Microbial rhodopsins that are extremely distantly related to animal visual rhodopsins comprise an expansive family of seven transmembrane proteins that contain a covalently attached cofactor, retinal. Upon absorption of a photon, retinal isomerizes triggering a series of structural transformations that correlate with functional and spectral changes and are known as the photocycle. Here we present a structural and functional characterization of Organic Lake Phycodnavirus rhodopsin II (OLPVRII), a representative of the second group of viral rhodopsins. Examination of the crystal structure, functional characterization and molecular dynamics (MD) simulations suggest that OLPVRII is a pentameric light-gated channel that is functionally analogous to well-studied pentameric ligand-gated ion channels playing crucial roles in many cellular processes.

The crystals diffracted up to 1.9 Å, and the structure of OLPVRII was solved at 1.9 Å. OLPVRII asymmetric unit cell contains five molecules of the protein organized in a pentamer with a bottle-like pore in the centre that has a narrow neck in the cytoplasmic part. Similarly to other microbial rhodopsins, each protomer of OLPVRII is organized as a bundle of seven transmembrane helices (A−G) connected by relatively short loops. The retinal cofactor is covalently bound to Lys195 through the Schiff base (RSB), and the electron densities indicate that the chromophore is in all-trans conformation. OLPVRII consists of only 211 amino acids and is the smallest among microbial rhodopsins with known crystal structure. Thus, the following amino acids play the key role in the formation of the pentamer: Glu26, Arg36, His37, Asn40, Trp203, and these amino acids are highly conserved within group II of viral rhodopsins, but not in other rhodopsins. The narrowest section (vestibule) of the pore is formed by the Phe24, Leu28 and Arg29 of helix A and has the length of 11 Å and mean diameter of 6 Å. Deeper into the pore, oxygen atoms of Leu28 main chain coordinate five water molecules forming a pentagon stabilized by hydrogen bonds with the mean distance between two neighboring molecules of 2.6 ± 0.2 Å (mean ± s.e.m., for different pentamer molecules). We assigned it to a short hydrocarbon chain that plugs the pore. In OLPVRII, the putative proton donor Glu42 is located in helix B (which corresponds to Thr46 in bR) and thus juxtaposed to the RSB.

>[4x]MSDLIEYSFYLTYAFLMTTGTITFIEALRTKNESVRHILNLETCISVVAAFFYSNFIGKLEHINYEEINLNRYVDWAITTPIMLLVLVLAFRVNQTNKAMVKFSDFMIILGMNYGMLGTGYLGDIGVIHKTMGTVLGFLFFGGLFYKLNTLRTSNASNDLLYGAFFVLWALYGVFYQMEQLPRNVGYNVLDLFSKCFVGIYFWAFYAKIFT;> MSDLIEYSFYLTYAFLMTTGTITFIEALRTKNESVRHILNLETCISVVAAFFYSNFIGKLEHINYEEINLNRYVDWAITTPIMLLVLVLAFRVNQTNKAMVKFSDFMIILGMNYGMLGTGYLGDIGVIHKTMGTVLGFLFFGGLFYKLNTLRTSNASNDLLYGAFFVLWALYGVFYQMEQLPRNVGYNVLDLFSKCFVGIYFWAFYAKIFTLEHHHHHH> GTEWKQGTEAAAVRSGDKVFFAGDSLMQGVAPFVQKSLKQQYGIESANLSKQSTGLSYPSFFDWPKTIEETLKKHPEISVLAVFLGPNDPWDFPVGKRYLKFASDEWAQE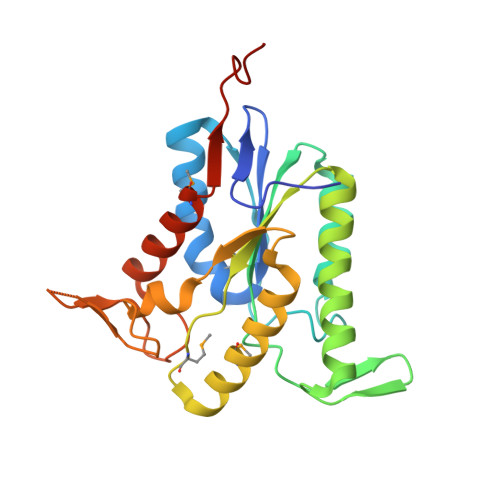YLKRVDRILEAAHTHRVQVVWLGIPYMKKVKLDGQMRYLDKLLSEHLKGKIILIPTAQTLSGGKGRYTDSVNVNGKPVRYRSKDGIHFTAEGQKLLAEKIMEKIVFEPSTQPSSTQP2-[2-[4-(4-methoxyphenyl)phenyl]sulfonylphenyl]ethanoic acid 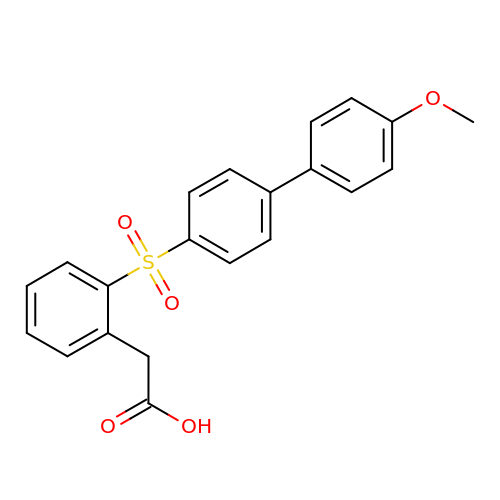| C21 H18 O5 S | FIPYOKGRSDJCAR-UHFFFAOYSA-N>[6x]MRTLLIRYILWRNDNDQTYYNDDFKKLML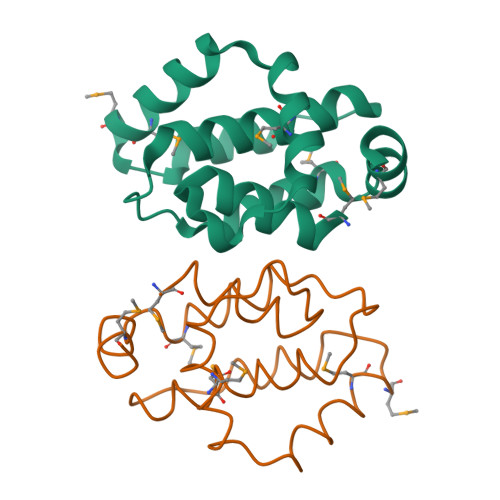LDELVDDGDVSTLIKNMRMTLSDGPLLDRLNQPVNNIEDAKRMIAISAKVARDIGERSEIRWEESFTILFRMIETYFDDLMIDLYGEK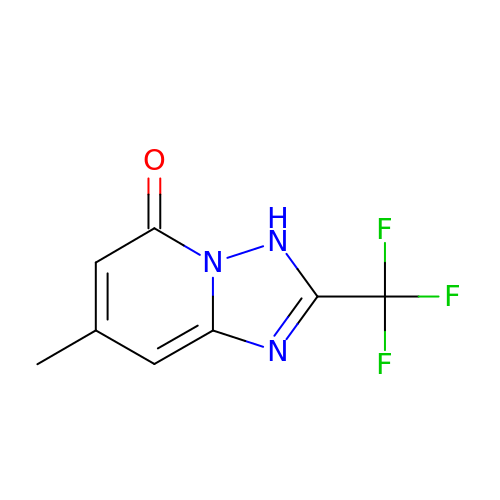7-methyl-2-(trifluoromethyl)-3~{H}-[1,2,4]triazolo[1,5-a]pyridin-5-one | C8 H6 F3 N3 O | DSCVNBORKMEUBZ-UHFFFAOYSA-N D-ribose | 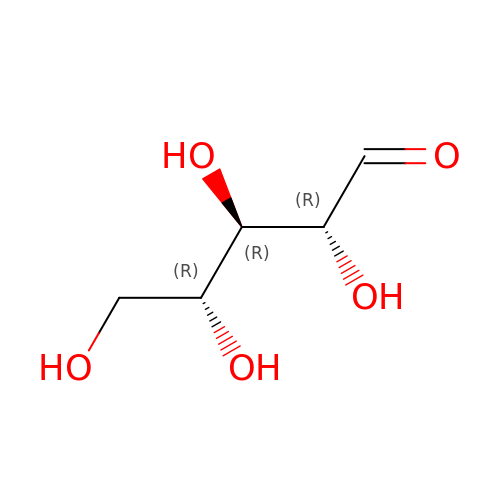C5 H10 O5 | PYMYPHUHKUWMLA-LMVFSUKVSA-N>[3x]MRVLLIAGGVSPEHEVSLLSAEGVLRHIPFPTDLAVIAQDGRWLLGEKALT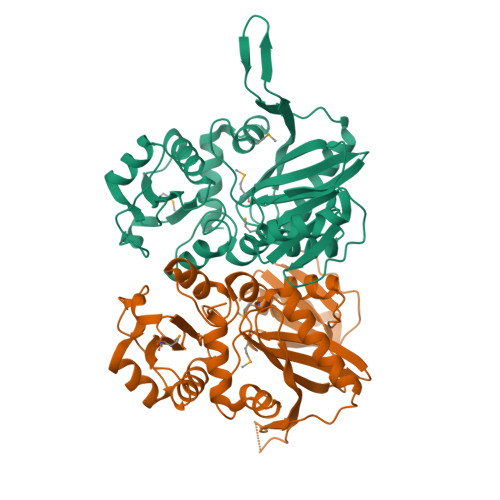ALEAKAAPEGEHPFPPPLSWERYDVVFPLLHGRFGEDGTVQGFLELLGKPYVGAGVAASALCMDKDLSKRVLAQAGVPVVPWVAVRKGEPPVVPFDPPFFVKPANTGSSVGISRVERFQDLEAALALAFRYDEKAVVEKALSPVRELEVGVLGNVFGEASPVGEVRYEAPFYDYETKYTPGRAELLIPAPLDPGTQETVQELALKAYKVLGVRGMARVDFFLAEGELYLNELNTIPGFTPTSMYPRLFEAGGVAYPELLRRLVELALT5-azanyl-3-[1-(pyridin-4-ylmethyl)indol-6-yl]-1~{H}-pyrazole-4-carbonitrile 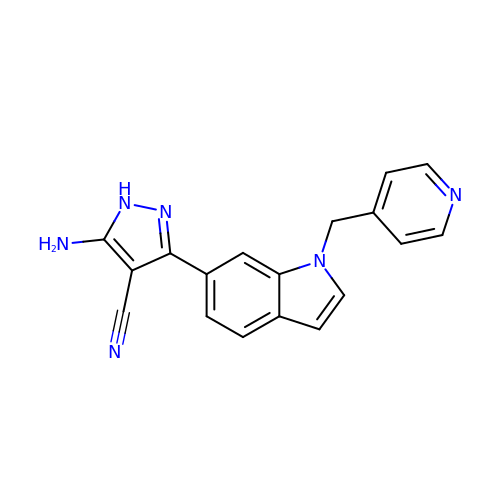| C18 H14 N6 | MOYIETQNOXXROV-UHFFFAOYSA-N> ETGQPAQCRIQKCTTDFVSLTSHLNSAVDGFDSEFCKALRAYAGCTQRTSKACRG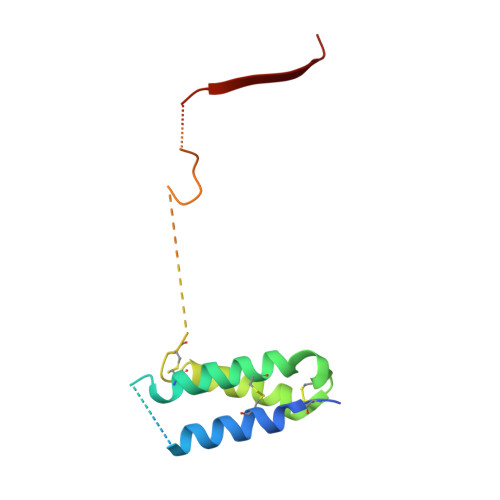NLVYHSAVLGISDLMSQRNCSKDGPTSSTNPEVTHDPCNYHSHAGAREHRRGDQNPPSYLFCGLFGD> TFEYGDGI;> HHHHHHHSSGLVPRGSHMAIYADNSYSIGNTPLVRLKHFGHNGNVVVKIEGRNPSYSVKCRIGANMVWQAEKDGTLTKGKEIVDATSGNTGIALAYVAAARGYKITLTMPETMSLERKRLLCGLGVNLVLTEGAKGMKGAIAKAEEIVASDPSRYVMLKQFENPANPQIHRETTGPEIWKDTDGKVDVVVAGVGTGGSITGISRAIKLDFGKQITSVAVEPVES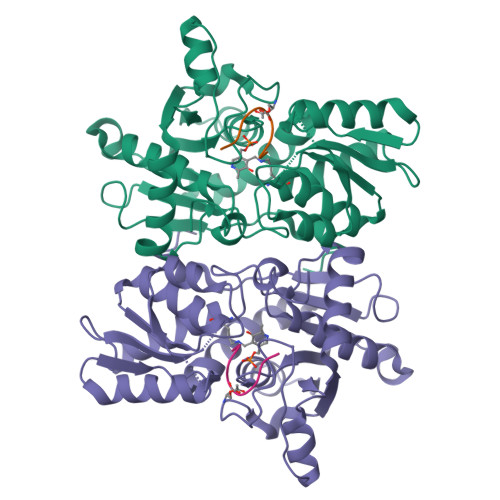PVISQTLAGEEVKPGPHKIQGIGAGFIPKNLDLSIIDRVETVDSDTALATARRLMAEEGILAGISSGAAVAAADRLAKLPEFADKLIVVILPSASERYLSTALFEGIEG> KS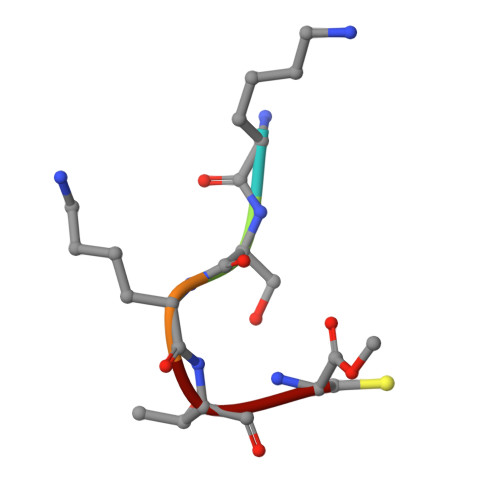KTC>[2x]APVCGVRASGRVCPDGYCCSQWGYCGTTEEYCGKGCQSQCDYNRCGKEFGGKECHDELCCSQYGWCGNSDGHCGEGCQSQCSYWRCGKDFGG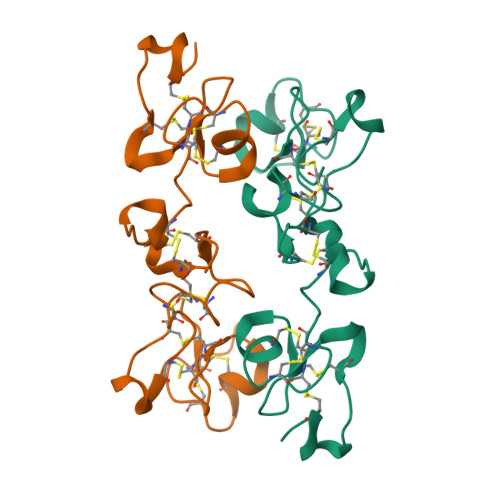RLCTEDMCCSQYGWCGLTDDHCEDGCQSQCDLPT>[2x]MMVLVSYDVSTSSPGGDKRLRKVAKACRDLGQRV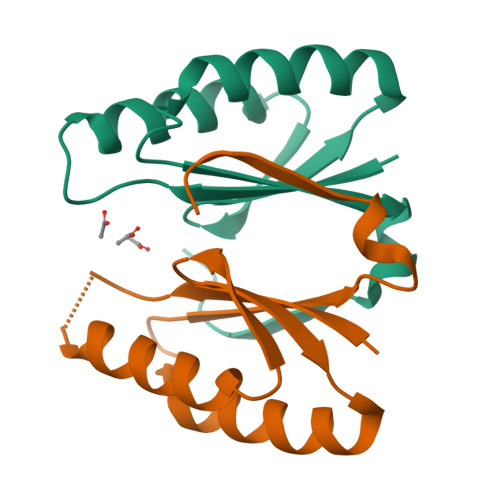QFSVFEIEVDPAQWTALRQRLCDLIDPDIDSLRFYHLGAKWEARVEHVGAKPSLDLKGPLIFLEHHHHHH>[2x]MEPLDELDLLLLEEDGGAEAVPRVELLRKKADALFPETVLSRGVDNRYLVLAVETSQNERGAEEKRLHVTASQDREHEVLCILRNGWSSVPVEPGDIVHLEGDCTSEPWIIDDDFGYFILYPDMMISGTSVASSIRCLRRAVLSETFRGSDPATRQMLIGTILHEVFQKAISESFAPERLQELALQTLREVRHLKEMYRLNLSQDEILCEVEEYLPSFSKWAEDFMRKGPSSEFPQMQLSLPSDGSNRSSPCNIEVVKSLDIEESIWSPRFGLKGKIDVTVGVKIHRDCKMKYKVMPLELKTGKESNSIEHRSQVVLYTLLSQERREDPEAGWLLYLKTGQMYPVPANHLDKRELLKLRNWLAASLLHRVSRAAPGEEARLSALPQIIEEEKTCKYCSQIGNCALYSRAVEEQGDDASIPEAMLSKIQEETRHLQLAHLKYFSLWCLMLTLESQSKDNRKTHQSIWLTPASELEESGNCVGNLVRTEPVSRVCDGQYLHNFQRKNGPMPATNLMAGDRIILSGEERKLFALSKGYVKKMNKAAVTCLLDRNLSTLPATTVFRLDREERHGDISTPLGNLSKLMESTDPSKRLRELIIDFREPQFIAYLSSVLPHDAKDTVANILKGLNKPQR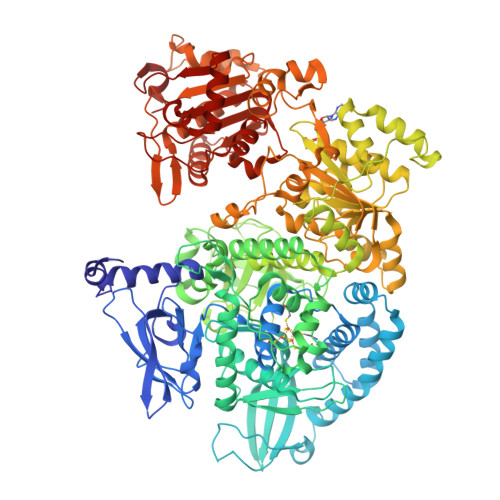QAMKRVLLSKDYTLIVGMPGTGKTTTICALVRILSACGFSVLLTSYTHSAVDNILLKLAKFKVGFLRLGQSHKVHPDIQKFTEEEICRSRSIASLAHLEELYNSHPIVATTCMGINHPIFSRKTFDFCIVDEASQISQPVCLGPLFFSRRFVLVGDHQQLPPLVVNREARALGMSESLFKRLERNESAVVQLTVQYRMNRKIMSLSNKLTYAGKLECGSDRVANAVLALPNLKDARLSLQLYADYSDSPWLAGVLEPDNPVCFLNTDKVPAPEQVENGGVSNVTEARLIVFLTSTFIKAGCSPSDIGVIAPYRQQLRIISDLLARSSVGMVEVNTVDKYQGRDKSLILVSFVRSNEDGTLGELLKDWRRLNVALTRAKHKLILLGSVSSLKRFPPLGTLFDHLNAEQLILDLPSREHESLSHIL>GHHHHHHELANNTTGFTRIIKAAGYSWKGLRAAWINEAAFRQEGVAVLLAVVIACWLDVDAITRVLLISSVMLVMIVEILNSAIEAVVDRIGSEYHELSGRAKDMGSAAVLIAIIVAVI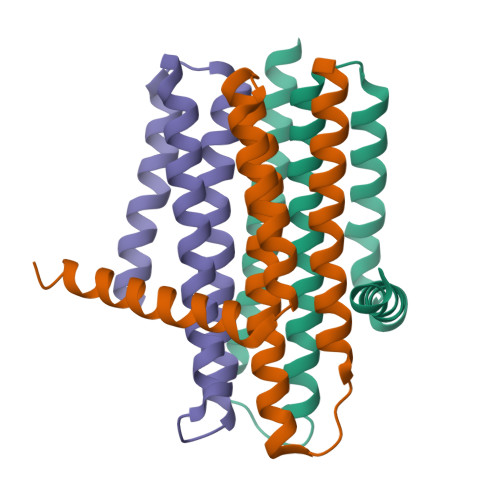TWCILLWSHFG[3x]> GAQVSRQNNGTHENGVTASNGSVIKYFNINYYKDSASSGLSRQDFSQDPSKFTQPLV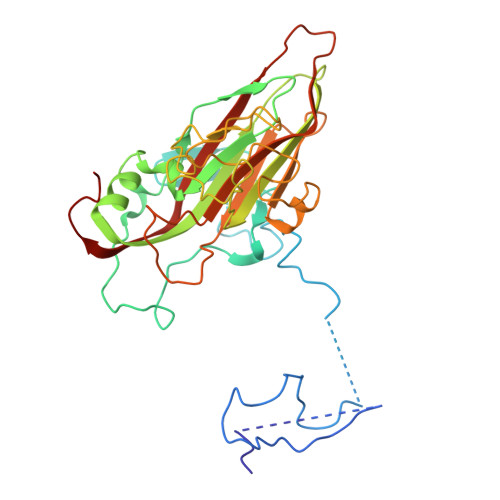DTLTNPALMSPSVEACGYSDRLKQITIGNSTITTQDSLHTVLAYGEWPTYLSDIDATSVDKPTHPETSADRFYTLDSVEWQVGSHGWWWKLPDALKDMGVFGQNMYYHSMGRSGFIIHTQCNATKFHSGALIVAVIPEHQLAYVGGVKVNVGYDHTHPGQSGHQIRGPSQSNDRSGGKPDEDPLFNCNGTLLGNITIFPHQIINLRTNNSSTIVVPYINCVPMDNMLKHNNLSLVIIPLVPLRPGSSGINSVPITVTIAPYKSEFSGAMEAQRQ>MNAIADVQSSRDLRNLPINQVGIKDLRFPITLKTAEGTQSTVARLTMTVYLPAEQKGTHMSRFVALMEQHTEVLDFAQLHRLTAEMV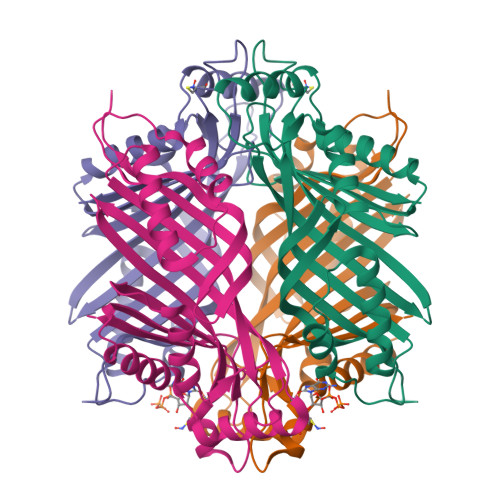ALLDSRAGKISVSFPFFRKKTAPVSGIRSLLDYDVSLTGEMKDGAYGHSMKVMIPVTSLCPCSKEISQYGAHNQRSHVTVSLTSDAEVGIEEVIDYVETQASCQLYGLLKRPDEKYVTEKAYENPKFVEDMVRDVATSLIADKRIKSFVVESENFESIHNHSAYAYIAYP[2x]One of the most important virulence factors of B. pertussis and an obvious target for improving current aP vaccines is pertussis toxin (PTx). This exotoxin is a multimeric, 105 kDa protein, composed of five subunits arranged in a typical A–B structure. PTx is an ADP-ribosylase that catalyzes the transfer of an ADP-ribose group from an NAD+ substrate to a cysteine residue of the α-subunit of the trimeric GTP-binding protein (G protein). Ribosylation of these G proteins impairs the binding of G proteins to the G protein-coupled receptor, on the host cell membrane, promoting adenylate cyclase activity that causes an increase in the intracellular levels of cAMP.

From these, a variant with a double mutation in the S1 subunit substituting Arg9 by Lys and Glu129 by Gly (PT-9K/129G) has been shown to completely abolish the toxic effects and has displayed the lowest enzymatic activity of the many variants generated. In addition, the space group between PTx and gdPT was the same with nearly identical cell dimensions and crystal packing interfaces. Despite the minor differences observed between gdPT and the previously reported PTx structural data, the double mutation (R9K/E129G) in the catalytic site of subunit S1 (the A-domain) does not appear to affect the overall folding of the protein. In PTx, Arg9 forms hydrogen bonding interactions with Ser52 and Asp11. The incorporation of Lys in position 9 maintains the hydrogen bonding with Ser52; however, it induced substantial changes in the hydrogen bonding network. When examining the effect of the E129G substitution, all interactions at position 129 (His35, as well as the hydrogen bonding with Gln127) were lost. The changes in the hydrogen bonding network due to either R9K or E129G mutations did not modify the shape of the catalytic pocket. These results indicate that the double mutation does not alter the overall architecture of the active site, despite changes in the hydrogen bonding network surrounding Arg9 and Gly129 residues. Regions with increased deuterium uptake are more solvent accessible (red); this is a result of either greater structural flexibility in the protein sequence or changes in protein conformation. Since the crystal structure of gdPT did not show any differences in protein conformation, it can be inferred that the R9K and E129G mutations result in increased conformational flexibility in the catalytic core of the subunit. The rigidification of this mobile loop, along with increased flexibility in the catalytic cleft are predicted to impair NAD+ binding within the catalytic site.

>[2x]MRCTRAIRQTARTGWLTWLAILAVTAPVTSPAWADDPPATVYKYDSRPPEDVFQNGFTAWGNNDNVLEHLTGRSCQVGSSNSAFVSTSSSRRYTEVYLEHRMQEAVEAERAGRGTGHFIGYIYEVRADNNFYGAASSYFEYVDTYGDNAGRILAGALATYQSGYLAHRRIPPENIRRVTRVYHNGITGETTTTEYSNARYVSQQTRANPNPYTSRRSVASIVGTLVRMAPVVGACMARQAESSEAMAAWSERAGEAMVLVYYESIAYSF;>MPIDRKTLCHLLSVLPLALLGSHVARASTPGIVIPPQEQITQHGSPYGRCANKTRALTVAELRGSGDLQEYLRHVTRGWSIFALYDGTYLGGEYGGVIKDGTPGGAFDLKTTFCIMTTRNTGQPATDHYYSNVTATRLLSSTNSRLCAVFVRSGQPVIGACTSPYDGKYWSMYSRLRKMLYLIYVAGISVRVHVSKEEQYYDYEDATFETYALTGISICNPGSSLC[2x];>[2x]MLINNKKLLHHILPILVLALLGMRTAQAVAPGIVIPPKALFTQQGGAYGRCPNGTRALTVAELRGNAELQTYLRQITPGWSIYGLYDGTYLGQAYGGIIKDAPPGAGFIYRETFCITTIYKTGQPAADHYYSKVTATRLLASTNSRLCAVFVRDGQSVIGACASPYEGRYRDMYDALRRLLYMIYMSGLAVRVHVSKEEQYYDYEDATFQTYALTGISLCNPAASIC;>MLRRFPTRTTAPGQGGARRSRVRALAWLLASGAMTHLSPALADVPYVLVKTNMVVTSVAMKPYEVTPTRMLVCGIAAKLGAAASSPDAHVPFCFGKDLKRPGSSPMEVMLRAVFMQQRPLRMFLGPKQLTFEGKPALELIRMVECSGKQDCP[4x];>MQRQAGLPLKANPMHTIASILLSVLGIYSPADVAGLPTHLYKNFTVQELALKLKGKNQEFCLTAFMSGRSLVRACLSDAGHEHDTWFDTMLGFAISAYALKSRIALTVEDSPYPGTPGDLLELQICPLNGYCE[2x]> MFVEVDESKIKPKYAREDVVASACKQFEFRPDLAATSIRTAFVLAARR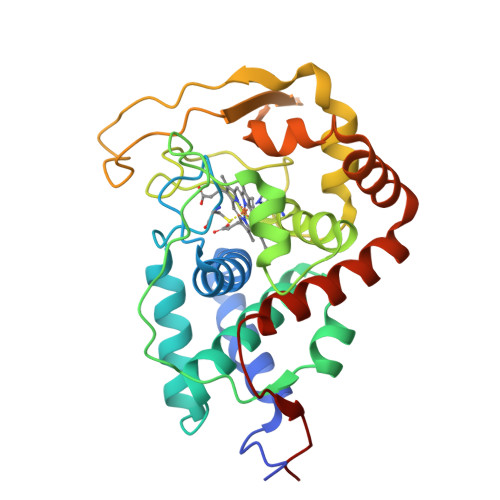AGFPAETVDESCAVVRGLDDVAGIMNYLSSTYPASSTEDVASLAAIAGIKYLNGPYEAILDQWRWGRNDSDTAPTRNIPKNPNQNVFSIPTILHALGGLTEAECVALLACHSVGEFHENVSGLESATHTGRRYTLNNRYYQFLLEHERAFAPLTVARTQYNKEVATLPQTLRCVYVKENTNGKAKKRQCVVNAAELELLKNKTWRELVVRYAADEELWREQFQSAFTKMIESNFKRLRPYSDPNSA>MVSKGEEDNMASLPATHELHIFGSINGVDFDMVGQGTGNPNEGYEELNLKSTKGDLQFSPWILVPHVGWGFHQYLPYPDGMSPFQAAMVDGSGYQVHRTMQFEDGASLTVNYRYTYEGSHIKGEAQVKGTGFPADGPVMTNSLTAVDSCWSKKTYPNDKTIISTFKWSYTTGNGERYRSTARTTYTFAKPMAANYLKNQPVYVFRKTELKHSETELN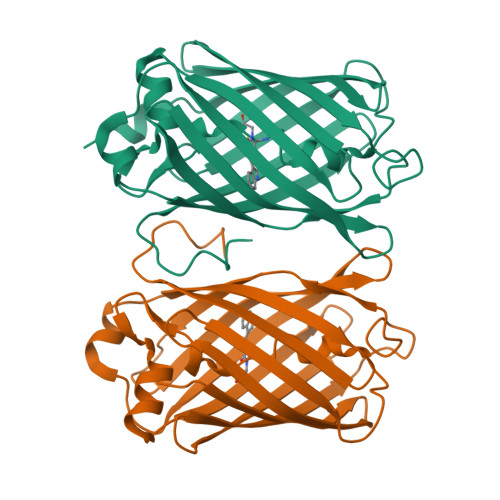FKEWQKAFTDVMGMDELYK[4x]> MRGSHHHHHHGSRMLSRYEKWEKIKQHYQHWSDSLSEEGRGLLKKLQIPIEPKKDDIIHSLSQEEKELLKRIQIDSSDFLSTEEKEFLKKLQIDIRDSLSEEEKELLNRIQVDSSNPLSEKEKEFLKKLKLDIQPYDINQRLQDTGGLIDSPSINLDVRKQYKRDIQNIDALLHQSIGSTLYNKIYLYENMNINNLTATLGADLVDSTDNTKINRGIFNEFKKNFKYSISSNYMIVDINERPALDNERLKWRIQLSPDTRAGYLENGKLILQRNIGLEIKDVQIIKQSEKEYIRIDAKVVPKSKIDTKIQEAQLNINQEWNKALGLPKYTKLITFNVHNRYASNIVESAYLILNEWKNNIQSDLIKKVTNYLVDGNGRFVFTDITLPNIAEQ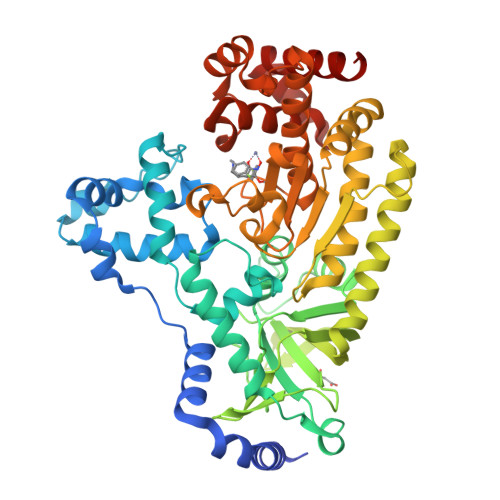YTHQDEIYEQVHSKGLYVPESRSILLHGPSKGVELRNDSEGFIHEFGHAVDDYAGYLLDKNQSDLVTNSKKFIDIFKEEGSNLTSYGRTNEAEFFAEAFRLMHSTDHAERLKVQKNAPKTFQFINDQIKFIINS>[2x]GSHMDSTTIQQNKDTLSQIVVFPTGNYDKNEANAMVNRLANIDGKYLNALKQNNLKIKLLSGKLTDEKEYAYLKGVV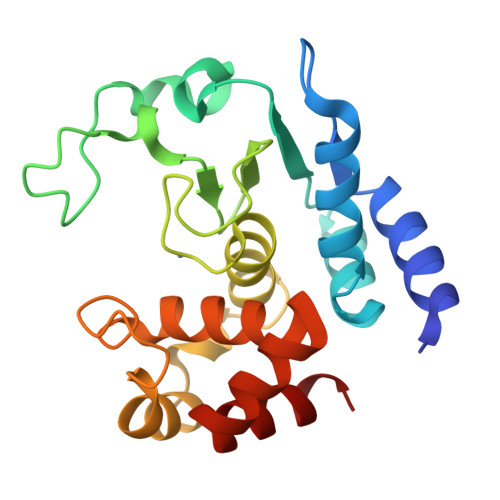PKGWEGTGKTWDDVPGLGGSTVALRIGFSNKGKGHDAINLELHATAHAIDHIVLNDISKSAQFKQIFAKEGRSLGNVNYLGVYPEEFFAESFAYYYLNQDTNSKLKSACPQTYSFLQNLAK> MDAPVTPYIWQYQPQTGKAAGARQNYGAVINWLSADNNMFHRVQTVNRARNLIDEIREETVRPDLAASFNDWTYDQLTQPPGTAYLPAPDPLTGPTTIRDKVLSAEGEQLAGSRPSVLHGGASLPPSAYSLGDGREYMKLTRDALPFPQNWMVKENGVWTPIVEQRAALRGGSANALSSYPTLLFNQPPILRYRRPGQQLQGSGVIAPSSKVLSLLSEAPRIPRTEGMTPYQFANSFPPVVYEDPFSQNLAVFPKEFSPLFEPENQVLASSLA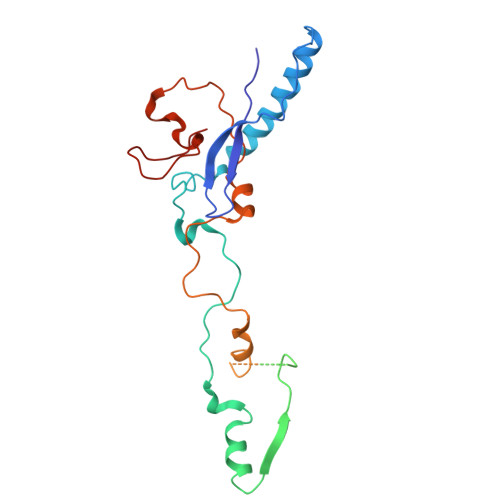TLQYN> MAKLNMNNEIKKVEQRLEKAIKSKDSVLEQASLHLLSSGGKRVRPAFVILSSQFGKDEQTSEQTYQVAVALELIHMATLVHDDVIDKSDKRRGKLTISKKWDQTTAILTGNFLLALGLEHLMAVKDNRVHQLISESIVDVCRGELFQFQDQFNSQQTIINYLRRINRKTALLIQISTEVGAITSQSDKETVRKLKMIGHYIGMSFQIIDDVLDFTSTEKKLGKPVGSDLLNGHITLPILLEMRKNPDFKLKIEQLRRDSERKEFEECIQIIRKSDSIDEAKAVSSKYLSKALNLISELPDG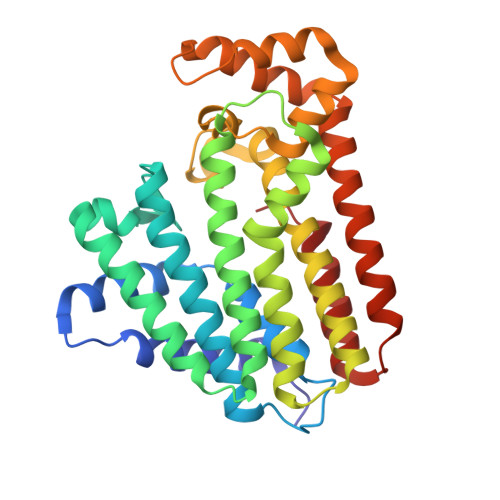HPKSLLLSLTKKMGSRNT> APSYPEYTREEVGRHRSPEERVWVTHGTDVFDVTDFVELHPGGPDKILLAAGGALEPFWALYAVHGEPHVLELLQQYKVGELSPDEAPAAPDAQDPFAGDPPRHPGLRVNSQKPFNAEPPAELLAERFLTPNELFFTRNHLPVPAVEPSSYRLRVDGPGGGTLSLSLAELRSRFPKHEVTATLQAAGNRRSEMSRVRPVKGLPWDIGAISTARWGGARLRDVLLHAGFPEELQGEWHVCFEGLDADPGGAPYGASIPYGRALSPAADVLLAYEMNGTELPRDHGFPVRVVVPGVVGARSVKWLRRVAVSPDESPSHWQQNDYKGFSPCVDWDTVDYRTAPAIQELPVQSAVTQPRPGAAVPPGELTVKGYAWSGGGREVVRVDVSLDGGRTWKVARLMGDKAPPGRAWAWALWELTVPVEAGTELEIVCKAVDSSYNV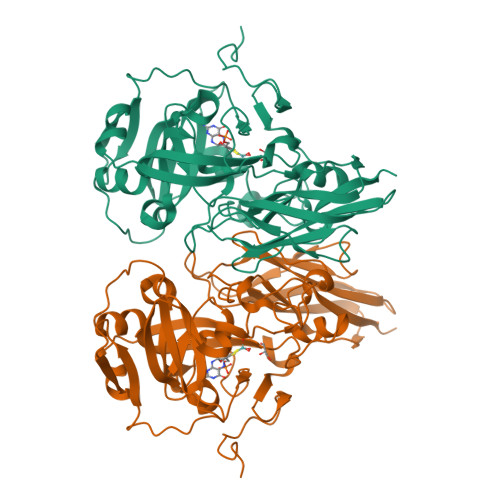QPDSVAPIWNLRGVLSTAWHRVRVSVQD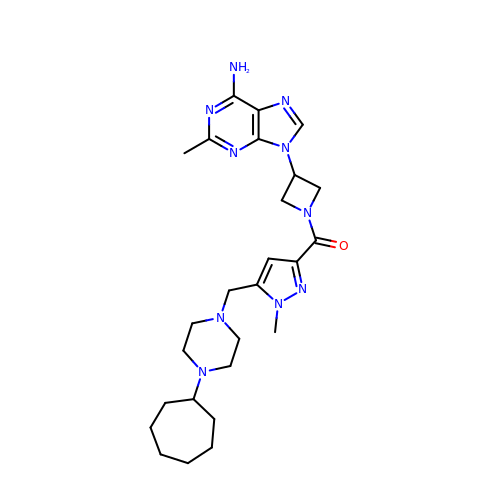[3-(6-amino-2-methyl-9H-purin-9-yl)azetidin-1-yl]{5-[(4-cycloheptylpiperazin-1-yl)methyl]-1-methyl-1H-pyrazol-3-yl}methanone | C26 H38 N10 O | YBGLVGMKTGYRQH-UHFFFAOYSA-N> GAMADDAAIQQTLAKMGIKSSDIQPAPVAGMKTVLTNSGVLYITDDGKHIIQGPMYDVSGTAPVNVTNKMLLKQLNALEKEMIVYKAPQEKHVITVFTDITCGY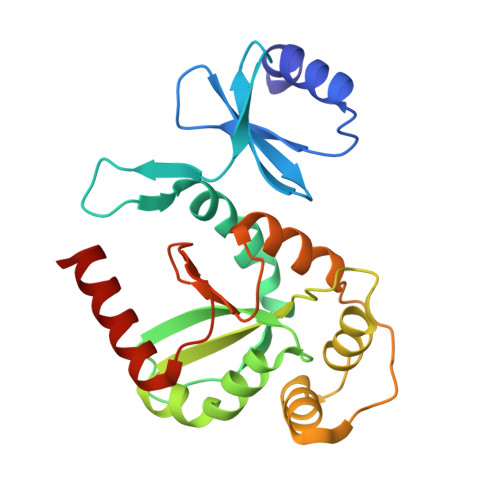SHKLHEQMADYNALGITVRYLAFPRQGLDSDAEKEMKAIWCAKDKNKAFDDVMAGKSVAPASCDVDIADHYALGVQLGVSGTPAVVLSNGTLVPGYQPPKEMKEFLDEHQKMTSGK> MKVHEIPRSQLLKIKQYEGSFVEWYRDLQEDRKKFASLLFRWAAFGYAAREDDGATYISPSQALLERRLLLGDAEDVAIKFLDVLFKGGAPSSSCYSLFYEDFALRDKAKYSGAKREFIEGLATMPLDKIIERIRQDEQLSKIPAEEWLILGAEYSPEEIWEQVAPRIVNVDRSLGKQLRERLGIKCRRPHDAGYCKILMEVVARQLRSHNETYHEYLNQTHEMKTKVANNLTNEFDLVCEFAEVLEEKNYGLGWYVLWQGVKQALKEQKKPTKIQIAVDQLRQPKFAGLLTAKWRALKGAYDTWKLKKRLEKRKAFPYMPNWDNDYQIPVGLTGLGVFTLEVKRTEVVVDLKEHGKLFCSHSHYFGDLTAEKHPSRYHLKFRHKLKLRKRDSRVEPTIGPWIEAALREITIQKKPNGVFYLGLPYALSHGIDNFQIAKRFFSAAKPDKEVINGLPSEMVVGAADLNLSNIVAPVKARIGKGLEGPLHALDYGYGELIDGPKILTPDGPRCGELISLKRDIVEIKSAIKEFKACQREGLTMSEETTTWLSEVESPSDSPRCMIQSRIADTSRRLNSFKYQMNKEGYQDLAEALRLLDAMDSYNSLLESYQRMHLSPGEQSPKEAKFDTKRASFRDLLRRRVAHTIVEYFDDCDIVFFEDLDGPSDSDSRNNALVKLLSPRTLLLYIRQALEKRGIGMVEVAKDGTSQNNPISGHVGWRNKQNKSEIYFYEDKELLVMDADEVGAMNILCRGLNHSVCPYSFVTKAPEKKNDEKKEGDYGKRVKRFLKDRYGSSNVRFLVASMGFVTVTTKRPKDALVGKRLYYHGGELVTHDLHNRMKDEIKYLVEKEVLARRVSLSDSTIKSYKSFAHV

Cas12h1 is a compact CRISPR-associated nuclease from functionally diverse type V CRISPR-Cas effectors and recognizes a purine-rich protospacer adjacent motif (PAM) distinct from that of other type V Cas effectors. Secondly, as a member of subtype V-H, Cas12h1 is distinguished by its relatively small size (870 amino acids), functioning as a compact DNA endonuclease guided by a single crRNA with proficient DNA cleavage capability, highlighting its potential as an efficient genome editing tool. Cas12h1 preferentially nicks the nontarget strand (NTS) of target dsDNA and indiscriminately cleaves ssDNA by collateral cleavage in the RuvC domain. Displaying a “Crab Claw” shape, Cas12h1 contains a distinguishable recognition (REC) lobe and a nuclease (NUC) lobe, with the two lobes connected by the WED domain.

We further reconstituted the wild-type Cas12h1-crRNA binary complex (hereafter termed the surveillance complex) to identify the activity of Cas12h1. To gain insight into the function of Cas12h1, we determined the structure of the surveillance complex using cryo-EM to a global resolution of 3.00 Å. Most residues of the PI domain (residues 103-173) are invisible in the surveillance complex, indicating its structural flexibility. The mature crRNA forms an elongated stem-loop structure containing a 36 nt repeat-derived sequence larger than other type V crRNAs (positions –35 to 0). The stem-loop structure is held upon the surface of the Helical II domain, with its 5’-end inserting into a positively charged groove formed by the WED domain, and is stabilized through numerous hydrogen bonds with Cas12h1. The density of nucleotides 6 to 26 in the spacer region of the crRNA was not observed, indicating its flexibility in the surveillance state. The surveillance structure revealed that the first 1-5 nucleotides of the crRNA were the pre-ordered seed sequences. A detailed analysis of the protein-crRNA interaction showed that nucleotide A(1) forms hydrogen bonds with the side chains of R8, Q688, R639. Although the lid motif (659–678 aa) is flexible in the surveillance state, structural superimposition of the motif suggested that the lid motif in the surveillance state clashes with the NTS in interference state at dT(13*), indicating that the lid motif sterically blocks the substrate from the catalytic site before target recognition. Specifically, the flexible lid motif is kept in an “off” conformation through hydrogen bonds between L660-E658, D659-V700, N671-L466, and L676-R634.> STAAVTGQTGLTITYPASA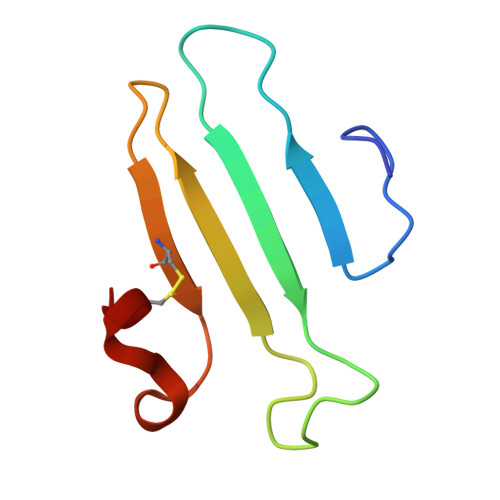TESAAIQGTFGNSAAIKIKNQTLTWTRTPEGAWSCATTVEAKFKPAGCAS> MKIATLFLALASSAAAFAPSQQVRSMTNEKMKPRQARNNFALNMKVDEMPGATAPLGKFDPLNLATLGSESTLAWFRAAELKHS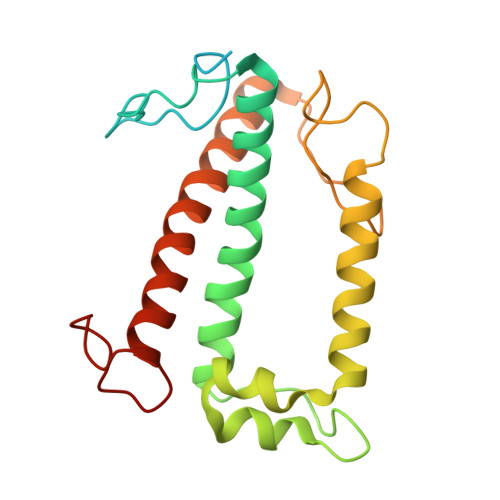RVAMLATTGYLVQAAGIHFPGMLSSDVSFESLSAMKPLDAWDAVPEGGKNQIYFTIFLAEFITECKGTHYTKGGPLPTIVFPPIDFSTVNPEQLKTRQNRELNNGRLAMIAIMSFVAAANIPGSVPALAGNPMF>[4x]MAGGRVRNIGDVMEHPLVELGVSYAALLSVIVVVVEYTMQLSGEYLVRLYLVDLILVIILWADYAYRAYKSGDPAGYVKKTLYEIPALVPAGLLALIEGHLAGLGLFRLVRLLRFLRILLIISRGSKFLSAIADAADKIRFYHLFGAVMLTVLYGAFAIYIVEYPDPNSSIKSVFDALWWAVVTATTVGYGDVVPATPIGKVIGIAVMLTGISALTLLIGTVSNMFQKILVGEPEPSSSPAKLAEMVSSMSEEEFEEFVRTLKNLRRLENSMKLVPRGSRSHHHHHH

KvAP is a Kv channel from the thermophilic archaea Aeropyrum pernix. All voltage sensors have a shared structure consisting of four helical transmembrane segments. The fourth helix, termed S4, contains positive-charged amino acids that move within the transmembrane electrical field as part of a global conformational change. Each subunit encodes a voltage sensor from transmembrane helices S1-S4 and one fourth of the pore from S5 and S6.

The final density map, calculated to 6 Å resolution, showed continuous density for the transmembrane region, density for the Fabs on the extracellular side and a poorly resolved cytoplasmic domain (CTD) on the intracellular side. An important first conclusion is that KvAP is a non-domain-swapped voltage-gated ion channel, meaning each voltage sensor is contiguous with the pore element from the same polypeptide chain. That this must be the case is evident in the short turn connecting S4 to S5 instead of a long α-helical S4-S5 linker. Therefore, KvAP is topologically like Kv10-12 channels and unlike Kv1-7 channels. In contrast, S1 in KvAP runs parallel to and in contact with S5 throughout its length inside the membrane. However, because of the unique interaction between S1 and S5, the S3b-S4 paddle in KvAP resides on the outer-most perimeter of the channel, oriented tangent to the pore domain. In the structure, the helical turn of S3b into S4, the Fab epitope, is exposed to the extracellular surface, compatible with Fab accessibility and a depolarized conformation of KvAP. The voltage sensor is similar in conformation to depolarized voltage sensors in other voltage-gated ion channels. The pore is less open than in the crystal structure of the full-length channel, but more open than in other closed K+ channels. The conformation of the inner helix gate in this structure might reflect a mixture of open and inactivated channels.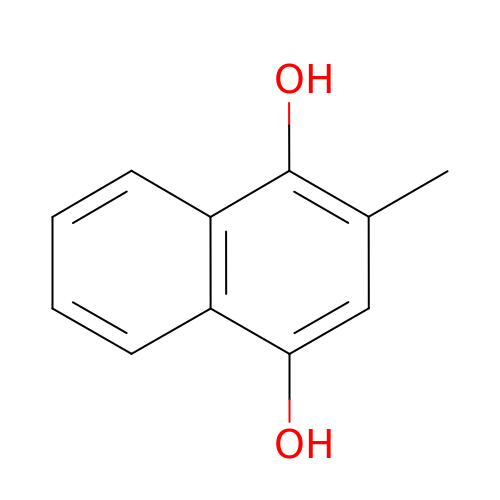2-methylnaphthalene-1,4-diol | C11 H10 O2 | ZJTLZYDQJHKRMQ-UHFFFAOYSA-N>SAASTLFVANLSAEVNEDTLRGVFKAFSGFTRLRLHNKNGSAVAFVEYSDLQKATQAMISLQGFQITANDRGGLRI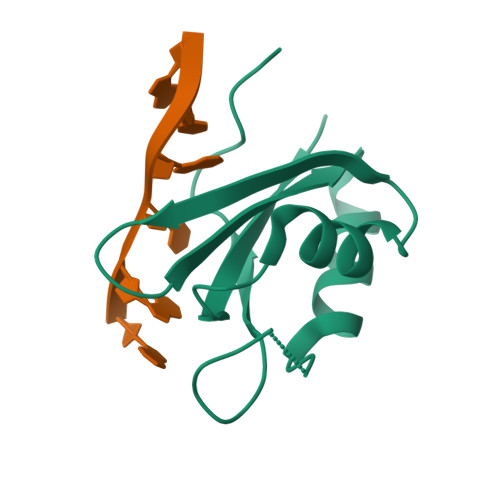EYARNKMADVNG[2x]>[2x]ENKFITKDDEVIDYIYGKISPLFALQYIRKIDLKHVFEYDY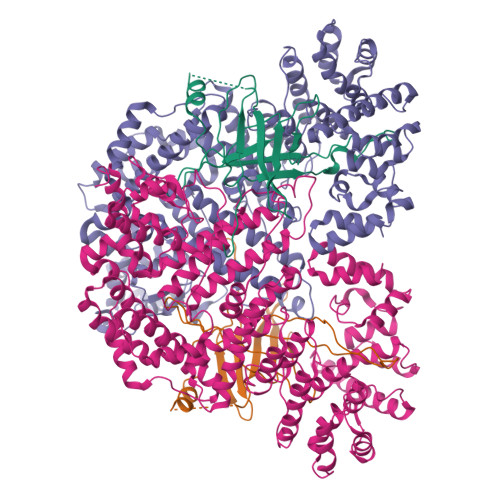HFEVNGTVVRHKNKGFGYMERFFELKESCDERSKLSKKQYERFNALFNFFEKNGVICMAKDAGTLNTSIEINSLAYHGKYDVMKKFIEEQSVSIEDDYKKAFFLACLGRWEESYDLYSNIILNSIDESNGCVYYLSQINRYRIYQSITQAVTQFNGLGLLTFGRHYKPFTDEFLARIEREMTNFNIDDLFNGMPFEFQKKYKILEFLSDNQFLYDDTVKLFELTNKVRSEMSEGSYSFGMSSDIVVLLRLYDNLRFLYENCLWSVSFHEFHQYIRNSMSLLIEKAEYERTRDIDELGFSFFGKKSGFFMEYYDFVNISRHFKIDDIKNLERSCSIDKIRFGEQEKIEEYLVGIAEEITKQFSANGMNVVFYTQFISEAKAALYFAKYVKLSEEGLGKIVKALLFYFPERDLDIGKRYVWLERLTKCNELPKSIISIIDDFLVLQAEKHIDQNYSEVSSNGLYSRDYGALIKHFEKNFISKRLSEITLCLTQDKQKQIDFLFKLLPLLSTNAKSHLLSFKSVENINDLMNGIRIGLIDEFTPEHEELIIEYLETRKVNYIVEKEKGIQTFSSNDYMSTFGIWYFLEEINNSKMEEFIGMDDQYDFFVDPENFDYKKFIPSWLKNYNDKLLGKIAGNKHMKHHVIEVLKERVKNSNDKRYLEILMNYFI;>MKTVIQDTADVYFKRKSDGKLVFTAEAQTASFSQAISEEKLRGGIGNKPLYILKSEKEINLTVKNAFFDLEWLAMTQGETIQEETKVKVFDREHGLIVDDTNKVTLKGKPVSDVTFYNKKGLTYKIAVSTDGTYTIPTAFAAAKDKLTAVYQIEKVGRRLAIKASKFSERYEVEYRTIAYNPDTEEVYSDIYIQFPNVSPSGEFEMSLENGNALAPEIKFEALADTDTDEMAVVIEASRDENTAAPVEDTTGSTQSSDLGGTTE[2x]(2E)-3-(4-hydroxy-3-methoxyphenyl)prop-2-enal | C10 H10 O3 | 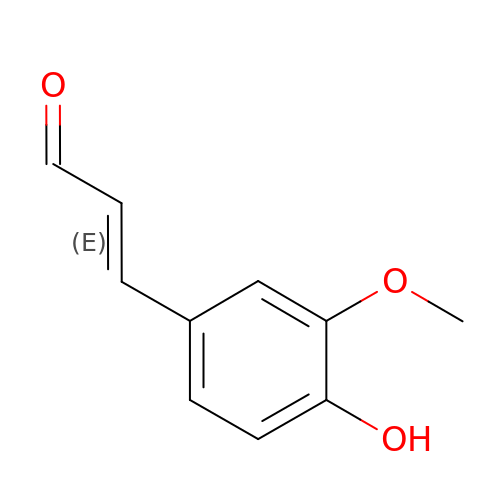DKZBBWMURDFHNE-NSCUHMNNSA-N> MVMDLGTTTIVAGQGDFSAYNYGNNGANWP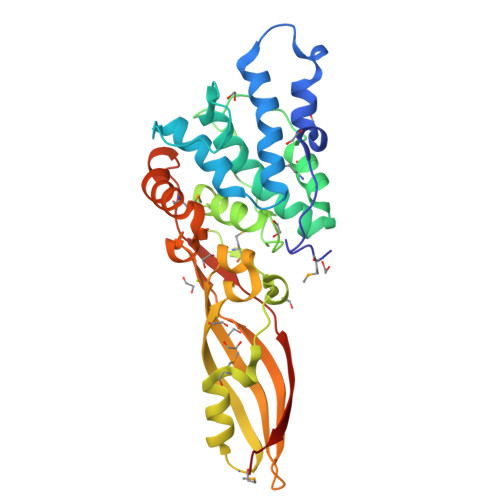APSPAQVGYISKGQRDVAYVNGDWEKPLLALWAQWANWGTTLYGYPSLPFPNYEFIWDIFDLPQADYNQFSLGDDRITAMNRAQNHQYPFPNNEGIPSWDRPKIDTFNGGVYTPAAAFAHYLTGKGKKMNFPIERLNIKPNVKAMPQFIGVLTSSPMGQTTVDFNVPYATAKDSWVAGNTVGEITLRIVGILVKSTSGQWSFRGEIRAYDDLYDFNPSNHRTETAEGMTRLGREVGQKFKDTTPYPIGIPGAIPVNISGRSHHHHHH>SSQLHVAIVSSPGMGHLIPVLVLGNRLATHHNIKITILAITTTSSSAETEFLKKTTLTNEEKTIEIIPVPSVDISHLINSSTKIFTQLRLLVREALPKIHSTIASMTHRPDALIVDIFCTQILPIAEEFNISKYTYHPTTAWTLALAIYCQVFDKEIEGEYVELKEPLKIPGCKALRPDDVVDPLLDRSDQQYEEYVKLGKEYTDFDGILINTWEDLEPETINALRYNEKLRLLLKVPVFPIGPLRRKVETTLNDEVIQWLDKQNNESVLFVSFGSGGTLSTKQMTELAWGLELSQQKFVWVVRPPSDGDADSAYLNSAGKDTRDMSEYLPEGFLTRTKDMGLVVPMWANQVEILSHSSVGGFLTHCGWNSTVESLTNGVPMIAWPLHAEQKMNAAMLTEELGVAIRPAVLPTKKLVKREEIQGMVRILMQTKEGKRIKEKAKKLKKSAENALSDGGSSYNSICELVKDIRSREL[2x]

NbUGT72AY1 is a promiscuous transferase that glycosylates bioactive hydroxycoumarins such as scopoletin and umbelliferone, as well as monolignols involved in lignin formation and various other small molecules. Five distinct GT protein folds have been identified that are capable of GT activity (termed GT-A to GT-E). NbUGT72AY1 adopts a GT-B fold comprised of two distinct N-terminal and C-terminal Rossmann-like domains (shown in cyan and brown in Fig. 2, respectively) of seven and six parallel β-sheets, respectively linked to α-helices, connected by a linker region and an interdomain cleft. The catalytic mechanism of inverting UGT such as NbUGT72AY1 is a direct displacement bimolecular nucleophilic substitution (SN2)-like reaction enabled by an enzymatic base catalyst.

Moreover, NbUGT72AY1 crystallized in the presence of scopoletin (III), UDP (IV), and a mixture of scopoletin and the non-transferable donor UDP2FG (V). Complex V and IV represent the SI and product-inhibited enzyme complexes, respectively, as they were obtained in the presence of an excess of substrate (scopoletin) and product (UDP), respectively. Asn372, Ser373, Glu376, Arg249, Ala351, and Trp350 frame their donor binding sites and in both structures, the indole ring of Trp350 points in the direction towards the uracil structure of UDP2FG and UDP, resulting in a π-stacking interaction. His18 is 4.0 Å apart from O7 of scopoletin in complex V and presumably plays the role of a catalytic base for the deprotonation of the acceptor to allow the nucleophilic attack at the anomeric centre of the donor. In NbUGT72AY1, Asp118 is located at a distance of 4.8 Å, while Tyr317, an amino acid of the closing loop, is only 2.8 Å apart. The product inhibited protein structure IV and SI complex V show closed active sites with distinct electron densities for the residues from 310-326 in IV and V, while catalytically active VI and VII lack electron densities for this region due to the high dynamics and the loop may remain open. The non-productive complexes IV and V are compact, fully resolved, and display a closed active site. Phe53, an amino acid of helix H2, interacts via π-cation binding with Arg214 of the UDPG-binding pocket and approaches Trp350 4.1 Å in SI complex V and 4.0 Å in the product-inhibited structure IV, while the distance is larger in all other structures. Although a ternary dead-end complex V was identified in our study, it differs from the previously postulated dead-end complex in that UDPG and not UDP is bound. Structures III and VII differ both in the length of helix H2 and in the spatial orientation of Trp350, leading to the formation of an unproductive SI complex V and a catalytically active complex VI, respectively, after binding of the respective second substrate.>M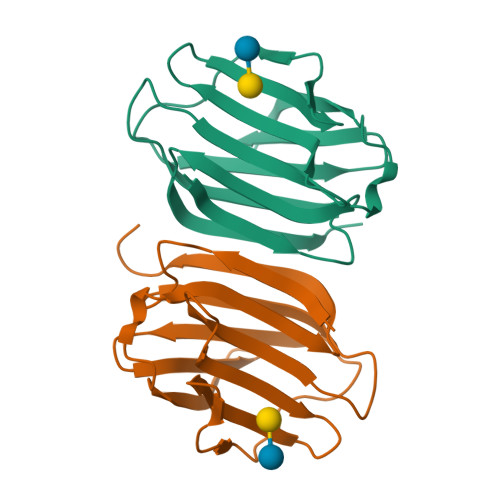ALRFEALYPEGMCPGWSVVVKGKTSSNTSMFEINFLSHPGDQIAFHFNPRFASSRIVCNSFLANHWGKEEVNKTFPFEAKEPFQVEIYSDQDYFHIFIDENKILQYKHRQKQLSSITKLQILNDIEISSVEITKRGLY[4x]> APLAVNDGDMRLADGGATNQGRVEIFYRGQWGTVCDNLWDLTDASVVCRALGFENATQALGRAAFGQGSGPIMLDEVQCTGTEASLADCKSLGWL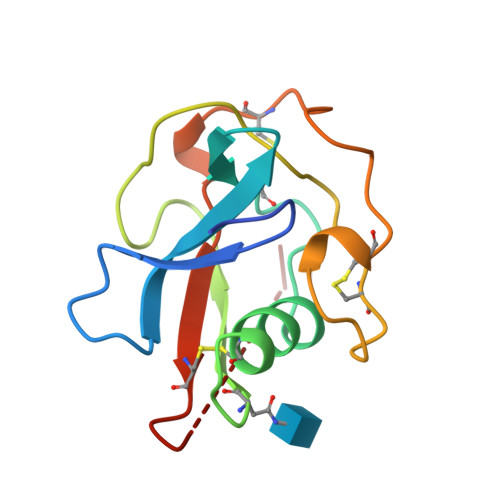KSNCRHERDAGVVCTNETRSTHTL>MRIGHGFDVHAFGGEGPIII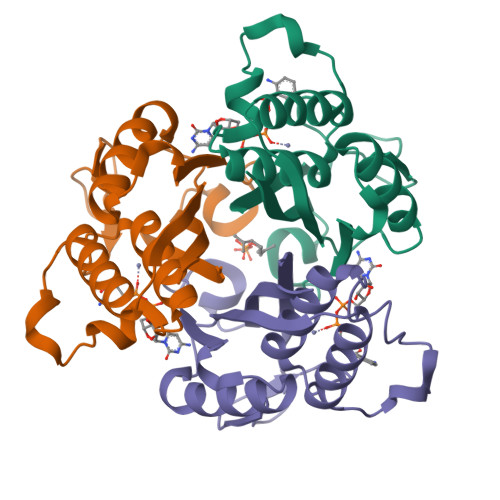GGVRIPYEKGLLAHSDGDVALHALTDALLGAAALGDIGKLFPDTDPAFKGADSRELLREAWRRIQAKGYTLGNVDVTIIAQAPKMLPHIPQMRVFIAEDLGCHMDDVNVKATTTEKLGFTGRGEGIACEAVALLIKATK[6x]>[4x]MVEATAQETDRPRFSFSI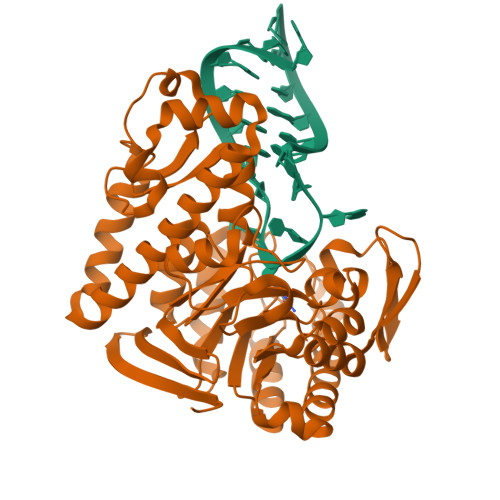AAREGKARTGTIEMKRGVIRTPAFMPVGTAATVKALKPETVRATGADIILGNTYHLMLRPGAERIAKLGGLHSFMGWDRPILTDSGGYQVMSLSSLTKQSEEGVTFKSHLDGSRHMLSPERSIEIQHLLGSDIVMAFDECTPYPATPSRAASSMERSMRWAKRSRDAFDSRKEQAENAALFGIQQGSVFENLRQQSADALAEIGFDGYAVGGLAVGEGQDEMFRVLDFSVPMLPDDKPHYLMGVGKPDDIVGAVERGIDMFDCVLPTRSGRNGQAFTWDGPINIRNARFSEDLKPLDSECHCAVCQKWSRAYIHHLIRAGEILGAMLMTEHNIAFYQQLMQKIRDSISEGRFSQFAQDFRARYFARNS> DSYTHLSFYEKRELFRKKLREIEGPEVTLVNEVDDEPCPSLDFQFISQYRLTQGVIPPDPNAQSGCNCSSLGGCDLNNPSRCECLDDLDEPTHFAYDAQGRVRADTGAVIYECNSACSCSMECPNRVVQRGRTLPLEIFKTKEKGWGVRSLR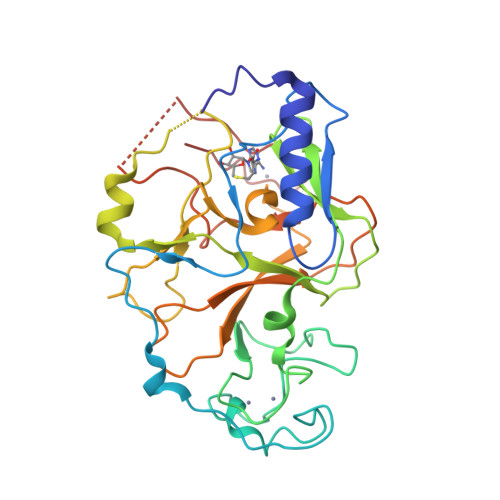FAPAGTFITCYLGEVITSAEAAKRDKNYDDDGITYLFDLDMFDDASEYTVDAQNYGDVSRFFNHSCSPNIAIYSAVRNHGARTIYDLAFFAIKDIQPLEELTFDYAGAKDFSPVQSQKSQQNRISKLRRQCKCGSANCRGWLFG;> SYTHLSFYEKRELFRKKLREIEGPEVTLVNEVDDEPCPSLDFQFISQYRLTQGVIPPDPNAQSGCNCSSLGGCDLNNPSRCECLDDLDEPTHFAYDAQGRVRADTGAVIYECNSACSCSMECPNRVVQRGRTLPLEIFKTKEKGWGVRSLRFAPAGTFITCYLGEVITSAEAAKRDKNYDDDGITYLFDLDMFDDASEYTVDAQNYGDVSRFFNHSCSPNIAIYSAVRNHGARTIYDLAFFAIKDIQPLEELTFDYAGAKDFSPVQSQKSQQNRISKLRRQCKCGSANCRGWLF>GSELRSIAFSRAVFAEFLATLLFVFFGLGSALNWPQALPSVLQIAMAFGLGIGTLVQALGHISGAHINPAVTVACLVGCHVSVLRAAFYVAAQLLGAVAGAALLHEITPADIRGDLAVNALSNSTTAGQAVTVELFLTLQLVLCIFASTDERRGENPGTPALSIGFSVALGHLLGIHYTGC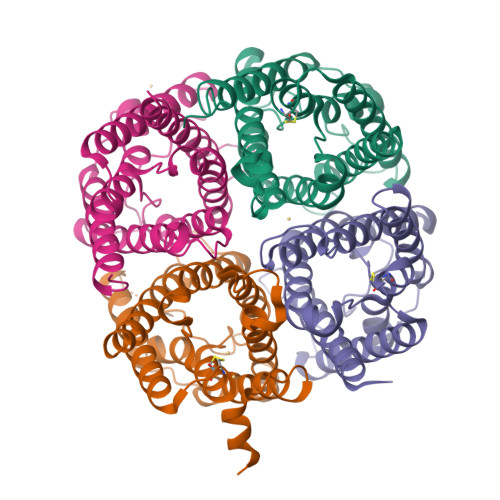SMNPARSLAPAVVTGKFDDHWVFWIGPLVGAILGSLLYNYVLFPPAKSLSERLAVLKGLEP[4x]>[2x]MELWLVRHGETLWNREGRLLGWTDLPLTAEGEAQARRLKGALPSLPAFSSDLLRARRTAEMAGFSPRLYPELR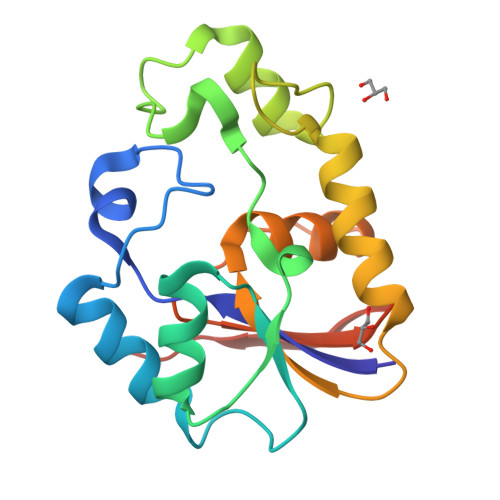EIHFGALEGALWETLDPRYKEALLRFQGFHPPGGESLSAFQERVFRFLEGLKAPAVLFTHGGVVRAVLRALGEDGLVPPGSAVAVDWPRRVLVRLALDGEEATG> GQNHHEVVKFMDVY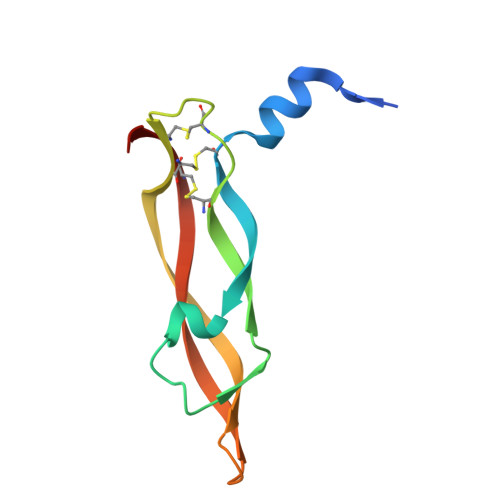QRSYCHPIETLVDIFQEYPDEIEYIFKPSCVPLMRCGGCCNDEGLECVPTEESNITMQIMRIKPHQGQHIGEMSFLQHNKCECRPKKD> MTDAKAFRRYIFELYFDPARLLELDDDQHLQRIERFLDALAPLHPVLENWYLCGDSLRDALSHNVTEHRQDLAKALSRDRRTRAVELVLWNGEEDPLKGGLSLDYEASGRAVSSRLQLEDAGSLLQVFDAPASSFVAIFLAVLEIWPETTWGMLAPHAYFVHQRTFPDRRSIGWIGFCPHPLRATDFPAATE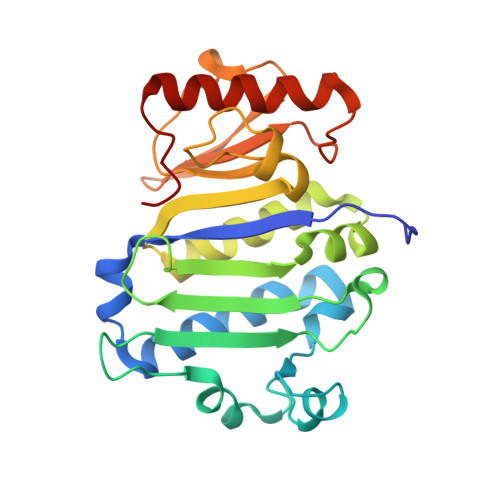LVDIPGRGTLLLNGREPMDETRREHFERVGEADIKLMELGYLPPLRG The respiratory syncytial virus (RSV) polymerase is a multifunctional RNA-dependent RNA polymerase composed of the large (L) protein and the phosphoprotein (P). It transcribes the RNA genome into ten viral mRNAs and replicates full-length viral genomic and antigenomic RNAs1. The RSV polymerase initiates RNA synthesis by binding to the conserved 3′-terminal RNA promoters of the genome or antigenome. The RSV L protein consists of five domains: the RdRp domain, the capping domain (Cap), the connector domain (CD), the methyltransferase domain (MT) and the carboxy-terminal domain (CTD).

The cryo-EM structure of the Le10-bound RSV polymerase revealed the presence of the RdRp and Cap domains of the L protein and the POD and PCTD domains of the P protein. In the Le10-bound RSV polymerase structure, the 3′ end of an incoming Le10 RNA template enters the template entrance channel, briefly touches the edge of the Cap domain, and runs towards the ‘GDN’ motif of the catalytic pocket from the bottom of the bowl. Additionally, the ‘priming loop’ (residues 1250–1280) of the Cap domain was distant from the active site, indicating that the structure represents a pre-initiation state for de novo RNA synthesis at position 3 of the template. Most of the interaction between Le10 RNA promoter and RSV L occurs at the ‘fingers’ (blue) and ‘peripheral’ (grey) regions, which form a composite tunnel for the RNA template to enter. The RNA–protein interactions can be divided into three parts: (I) positions 1–4 of Le10 and the catalytic pocket; (II) positions 5–7 of Le10 and the template entrance channel; (III) positions 8–10 of Le10 and the gate of the template entrance channel (Fig. 2a(I–III)). Specifically, the T1U backbone of Le10 interacts with the residue T660 from the supporting loop and K783 of the ‘palm’, contributing to the RNA template stability. No interaction was found between T2G and RSV L. Positions 3 and 4 of Le10 (T3C and T4G) are opposite to the catalytic residue D811, which occupies the −1 and +1 catalytic sites for RNA synthesis. The backbone of T3C interacts with residues K540, R637 and Q640 from the fingers region to stabilize the RNA template during initiation. The base of T4G interacts with residues K619, F629 and E778, all of which are conserved across the polymerases of NNS RNA viruses. The oxygen (O6) of the T4G base interacts with the nitrogen (NZ) of residue K619, and the nitrogen (N2) of the T4G base interacts with the oxygen (OE1) of residue E778. This may explain why RSV polymerase prefers a G at the +1 catalytic site for de novo RNA synthesis initiation, as G is the only base that contains an O atom towards K619 and an N atom towards E778. In the Le10-bound structure, there are twists at positions 5 and 8, followed by a 90° rotation for the bases of positions 8–10.

> MDPIINGNSANVYLTDSYLKGVISFSECNALGSYIFNGPYLKNDYTNLISRQNPLIEHMNLKKLNITQSLISKYHKGEIKLEEPTYFQSLLMTYKSMTSSEQIATTNLLKKIIRRAIEISDVKVYAILNKLGLKEKDKIKSNNGQDEDNSVITTIIKDDILSAVKDNQSHLKADKNHSTKQKDTIKTTLLKKLMCSMQHPPSWLIHWFNLYTKLNNILTQYRSNEVKNHGFTLIDNQTLSGFQFILNQYGCIVYHKELKRITVTTYNQFLTWKDISLSRLNVCLITWISNCLNTLNKSLGLRCGFNNVILTQLFLYGDCILKLFHNEGFYIIKEVEGFIMSLILNITEEDQFRKRFYNSMLNNITDAANKAQKNLLSRVCHTLLDKTVSDNIINGRWIILLSKFLKLIKLAGDNNLNNLSELYFLFRIFGHPMVDERQAMDAVKINCNETKFYLLSSLSMLRGAFIYRIIKGFVNNYNRWPTLRNAIVLPLRWLTYYKLNTYPSLLELTERDLIVLSGLRFYREFRLPKKVDLEMIINDKAISPPKNLIWTSFPRNYMPSHIQNYIEHEKLKFSESDKSRRVLEYYLRDNKFNECDLYNCVVNQSYLNNPNHVVSLTGKERELSVGRMFAMQPGMFRQVQILAEKMIAENILQFFPESLTRYGDLELQKILELKAGISNKSNRYNDNYNNYISKCSIITDLSKFNQAFRYETSCICSDVLDELHGVQSLFSWLHLTIPHVTIICTYRHAPPYIGDHIVDLNNVDEQSGLYRYHMGGIEGWCQKLWTIEAISLLDLISLKGKFSITALINGDNQSIDISKPIRLMEGQTHAQADYLLALNSLKLLYKEYAGIGHKLKGTETYISRDMQFMSKTIQHNGVYYPASIKKVLRVGPWINTILDDFKVSLESIGSLTQELEYRGESLLCSLIFRNVWLYNQIALQLKNHALCNNKLYLDILKVLKHLKTFFNLDNIDTALTLYMNLPMLFGGGDPNLLYRSFYRRTPDFLTEAIVHSVFILSYYTNHDLKDKLQDLSDDRLNKFLTCIITFDKNPNAEFVTLMRDPQALGSERQAKITSEINRLAVTEVLSTAPNKIFSKSAQHYTTTEIDLNDIMQNIEPTYPHGLRVVYESLPFYKAEKIVNLISGTKSITNILEKTSAIDLTDIDRATEMMRKNITLLIRILPLDCNRDKREILSMENLSITELSKYVRERSWSLSNIVGVTSPSIMYTMDIKYTTSTISSGIIIEKYNVNSLTRGERGPTKPWVGSSTQEKKTMPVYNRQVLTKKQRDQIDLLAKLDWVYASIDNKDEFMEELSIGTLGLTYEKAKKLFPQYLSVNYLHRLTVSSRPCEFPASIPAYRTTNYHFDTSPINRILTEKYGDEDIDIVFQNCISFGLSLMSVVEQFTNVCPNRIILIPKLNEIHLMKPPIFTGDVDIHKLKQVIQKQHMFLPDKISLTQYVELFLSNKTLKSGSHVNSNLILAHKISDYFHNTYILSTNLAGHWILIIQLMKDSKGIFEKDWGEGYITDHMFINLKVFFNAYKTYLLCFHKGYGKAKLECDMNTSDLLCVLELIDSSYWKSMSKVFLEQKVIKYILSQDASLHRVKGCHSFKLWFLKRLNVAEFTVCPWVVNIDYHPTHMKAILTYIDLVRMGLINIDRIHIKNKHKFNDEFYTSNLFYINYNFSDNTHLLTKHIRIANSELENNYNKLYHPTPETLENILANPIKSNDKKTLNDYCIGKNVDSIMLPLLSNKKLIKSSAMIRTNYSKQDLYNLFPMVVIDRIIDHSGNTAKSNQLYTTTSHQISLVHNSTSLYCMLPWHHINRFNFVFSSTGCKISIEYILKDLKIKDPNCIAFIGEGAGNLLLRTVVELHPDIRYIYRSLKDCNDHSLPIEFLRLYNGHINIDYGENLTIPATDATNNIHWSYLHIKFAEPISLFVCDAELSVTVNWSKIIIEWSKHVRKCKYCSSVNKCMLIVKYHAQDDIDFKLDNITILKTYVCLGSKLKGSEVYLVLTIGPANIFPVFNVVQNAKLILSRTKNFIMPKKADKESIDANIKSLIPFLCYPITKKGINTALSKLKSVVSGDILSYSIAGRNEVFSNKLINHKHMNILKWFNHVLNFRSTELNYNHLYMVESTYPYLSELLNSLTTNELKKLIKITGSLLYNFHNE;>[4x]MEKFAPEFHGEDANNRATKFLESIKGKFTSPKDPKKKDSIISVNSIDIEVTKESPITSNSTIINPTNETDDTAGNKPNYQRKPLVSFKEDPTPSDNPFSKLYKETIETFDNNEEESSYSYEEINDQTNDNITARLDRIDEKLSEILGMLHTLVVASAGPTSARDGIRDAMVGLREEMIEKIRTEALMTNDRLEAMARLRNEESEKMAKDTSDEVSLNPTSEKLNNLLEGNDSDNDLSLEDF> RSVPSSTILIPVVVHVVYNNSAQNISDAQIISQIQVLNEDFRRMNADQANTPSAFANLAGNANIEFKLARRDPNGNTTNGITRTSTSTETFSMEMDNVKFSNLGGNNAWNTRRYLNIWVCNLGDDLLGYAQFPFE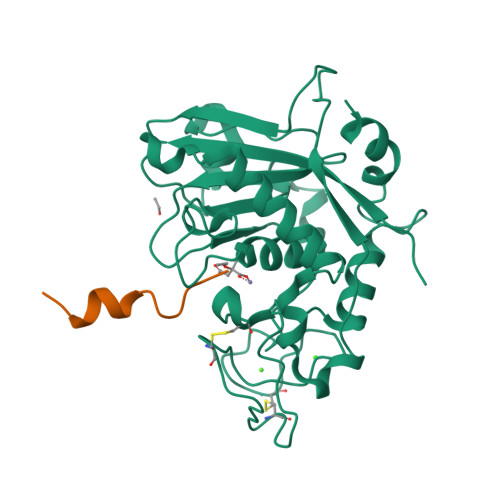FQTKPNTDGVVIHYKHFGRDGSAESPYDKGRTATHEVGHWLDLRHIWGDDGGSCSGTDNIADTPNQGGYNEGCPSFPKTDHCTNTSPGVMFMNYMDYTYDACMNLFTKGQVERMRSLFDTQTGIRREMQIYANELTNPLSFS;> KRDPVYFIKLSTIK>[4x]GKHYKRPQDELPCNEYSQPGGDGSYVSVPSPLGKIKSMTKEKADILLLRAGLPSHFHLQLSEIEFHEIIGSGSFGKVYKGRCRNKIVAIKRYRANTYCSKSDVDMFCREVSILCQLNHPCVIQFVGACLNDPSQFAIVTQYISGGSLFSLLHEQKRILDLQSKLIIAVDVAKGMEYLH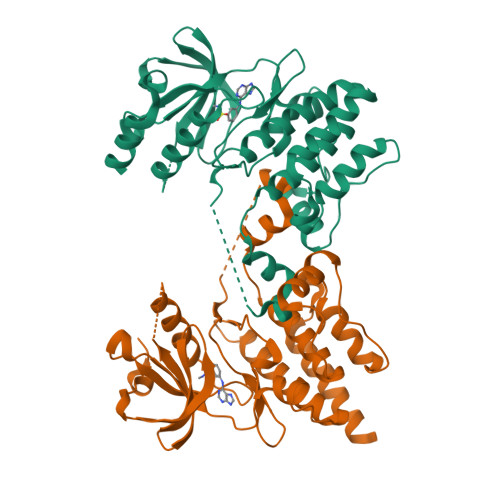NLTQPIIHRDLNSHNILLYEDGHAVVADFGESRFLQSLDEDNMTKQPGNLRWMAPEVFTQCTRYTIKADVFSYALCLWEILTGEIPFAHLKPAAADMDMAYHHIRPPIGYSIPKPISSLLIRGWNACPEGRPEFSEVVMKLEECLCNIELMS> GPGSMASDLFSQVVNSGPGSFLAKQLGVPQPETLRRYRPGDPPLAGSLLIGGSGRVAEPLRTALADDYNLVSNNIGGRWADSFGGVVFDATGITEAEGLKELYTFFTPLLRNLAPCARVVVVGTTPAEAGSVHAQVVQRALEGFTRSLGKELRRGATVSLVYLSADAKPGATGLESTMRFILSAKSAYVDGQVFRVGAADSTPPADWDKPLDGKVAVVTGAARGIGATIAEVFARDGATVVAIDVDGAAEDLKRVADKVGGTALTLDVTADDAVDKITAHVTEHHGGKVDILVNNAGI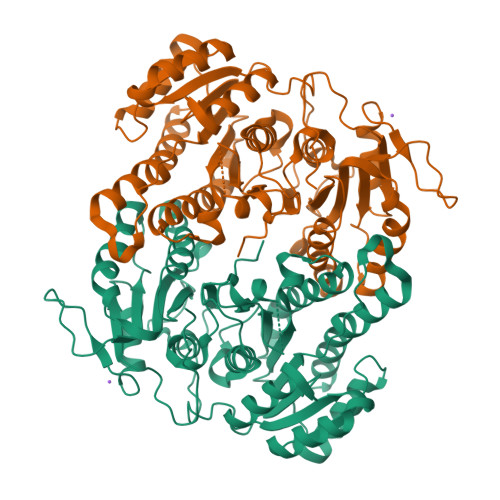TRDKLLANMDEKRWDAVIAVNLLAPQRLTEGLVGNGTIGEGGRVIGLSSMAGIAGNRGQTNYATTKAGMIGLAEALAPVLADKGITINAVAPGFIETKMTEAIPLATREVGRRLNSLFQGGQPVDVAELIAYFASPASNAVTGNTIRVCGQAMLGA>[3x]SMPKTISVRVTTMDAELEFAIQPNTTGKQLFDQVVKTIGLREVWFFGLQYQDTKGFSTWLKLNKKVTAQDVRKESPLLFKFRAKFYPEDVSEELIQDITQRLFFLQVKEGILNDDIYCPPETAVLLASYAVQSKYGDFNKEVHKSGYLAGDKLLPQRVLEQHKLNKDQWEERIQVWHEEHRGMLREDAVLEYLKIAQDLEMYGVNYFSIKNKKGSELWLGV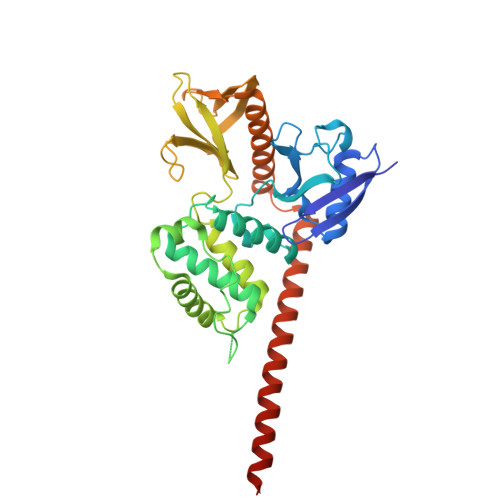DALGLNIYEQNDRLTPKIGFPWSEIRNISFNDKKFVIKPIDKKAPDFVFYAPRLRINKRIRALCMGNHELYMRRRKPDTIEVQQMKAQAREEKHQKQMERAMLENEKKKREMAEKEKEKIEREKEE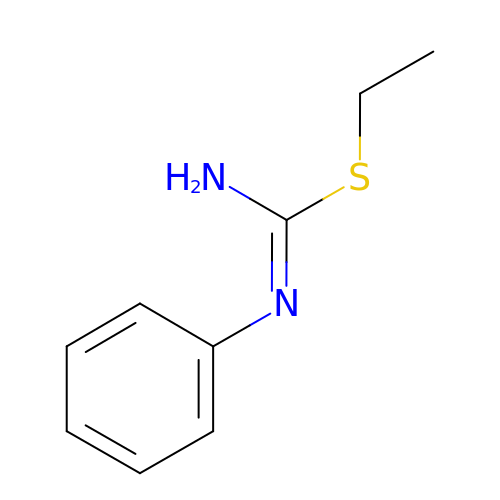2-ETHYL-1-PHENYL-ISOTHIOUREA | C9 H12 N2 S | LAXNJIWNBHHMDO-UHFFFAOYSA-N> AHHHHHHHRSDAAVIVVGAGPAGMMLAGELRLAGVEVVVLERLVERTGESRGLGFTARTMEVFDQRGILPRFGEVETSTQGHFGGLPIDFGVLEGAWQAAKTVPQSVTETHLEQWATGLGADIRRGHEVLSLTDDGAGVTVEVRGPEGKHTLRAAYLVGCDGGRSSVRKAAGFDFPGTAATMEMYLADIKGVELQPRMIGETLPGGMVMVGPLPGGITRIIVCERGTPPQRRETPPSWHEVADAWKRLTGDDIAHAEPVWVSAFGNATRQVTEYRRGRVILAGDSAHIHLPAGGQGMNTSIQDAVNLGWKLGAVVNGTATEELLDSYHSERHAVGKRLLMNTQAQGLLFLSGPEVQPLRDVLTELIQYGEVARHLAGMVSGLEITYDVGTGSHPLLGKRMPALELTTATRETSSTELLHTARGVLLDLADNPRLRARAAAWSDRVDIVTAVPGEVSATSGL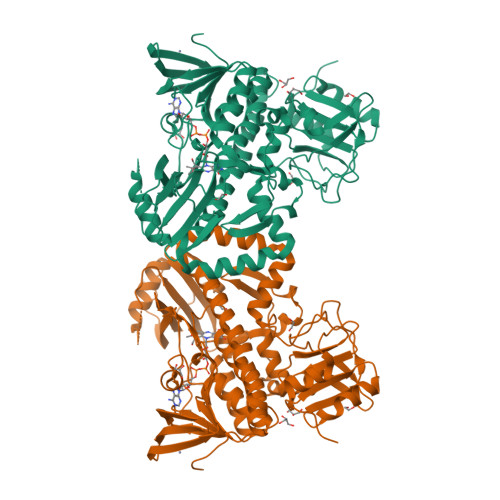RDTTAVLIRPDGHVAWAAPGSHHDLPMALERWFGAPLTG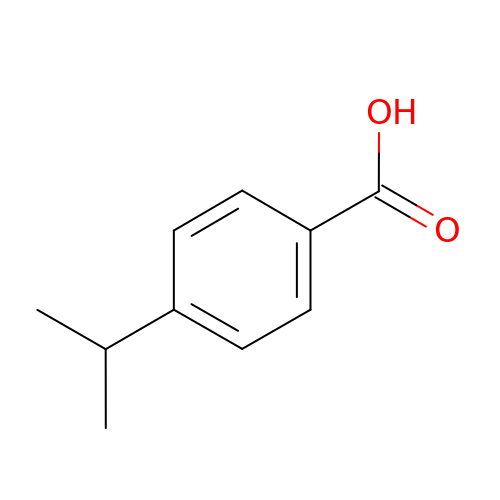4-propan-2-ylbenzoic acid | C10 H12 O2 | CKMXAIVXVKGGFM-UHFFFAOYSA-N> HHHHHHNRTVTVEELPIDPANVAAYAAVTGLRYGNQVPLTYPFALTFPSVMSLVTGFDFPFAAMGAIHTENHITQYRPIAVTDAVGVRVRAENLREHRRGLLVDL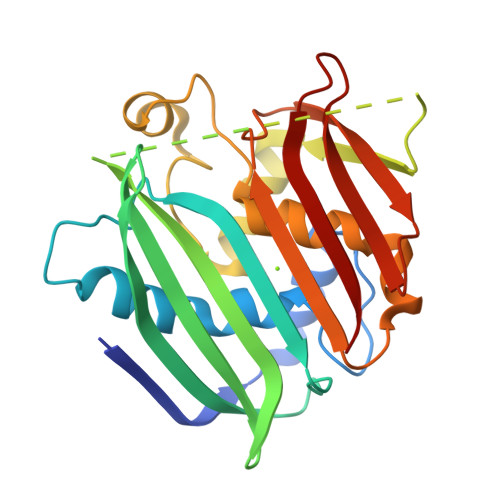VTNVSVGNDVAWHQVTTFLHQQRTSLSGEPKPPPQKKPKLPPPAAVLRITPAKIRRYAAVGGDHNPIHTNPIAAKLFGFPTVIAHGMFTAAAVLANIEARFPDAVRYSVRFAKPVLLPATAGLYVAEGDGGWDLTLRNMAKGYPHLTATVRGL>[2x]GMETVQLRNPPRRQLKKLDEDSLTKQPEE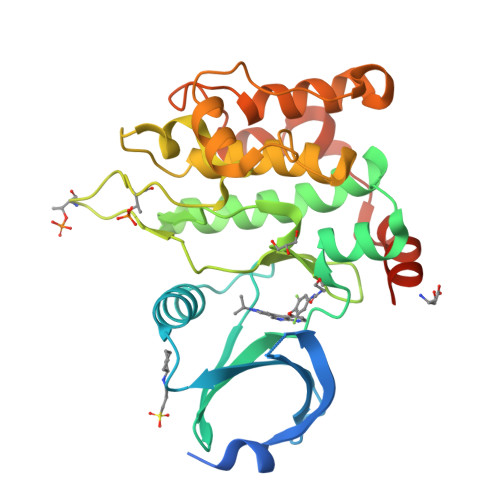VFDVLEKLGEGSYGSVYKAIHKETGQIVAIKQVPVESDLQEIIKEISIMQQCDSPHVVKYYGSYFKNTDLWIVMEYCGAGSVSDIIRLRNKTLTEDEIATILQSTLKGLEYLHFMRKIHRDIKAGNILLNTEGHAKLADFGVAGQLTDTMAKRNTVIGTPFWMAPEVIQEIGYNCVADIWSLGITAIEMAEGKPPYADIHPMRAIFMIPTNPPPTFRKPELWSDNFTDFVKQCLVKSPEQRATATQLLQHPFVRSAKGVSILRDLINEAMDVKLKRQESQQRE> MIRIENLSVSYKETLALKDISLVLHGPTITGIIGPNGAGK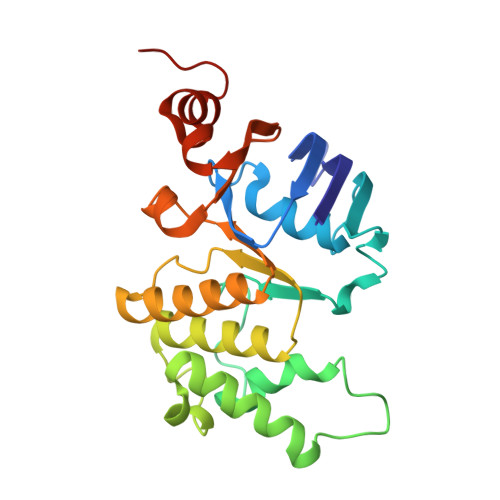STLLKGMLGIIPHQGQAFLDDKEVKKSLHRIAYVEQKINIDYNFPIKVKECVSLGLFPSIPLFRSLKAKHWKKVQEALEIVGLADYAERQISQLSGGQFQRVLIARCLVQEADYILLDEPFAGIDSVSEEIIMNTLRDLKKAGKTVLIVHHDLSKIPHYFDQVLLVNREVIAFGPTKETFTETNLKEAYGNQLFFNGGDL>[3x]GAMGMNTPPELDTVLQAPYAYNWPTSKNVKIASRIGIPYSTFQTIQPVSDAPNNGIGQITFNQPLGNLTGGAPRLRVSFTAEIKNILADSSLKDQIGLKSFPVNRSIPVAVINMNGKTFTSYPAQLIKLHQYNADPLELALLSPCSDVDEYNKIKAVSMNNPYRQ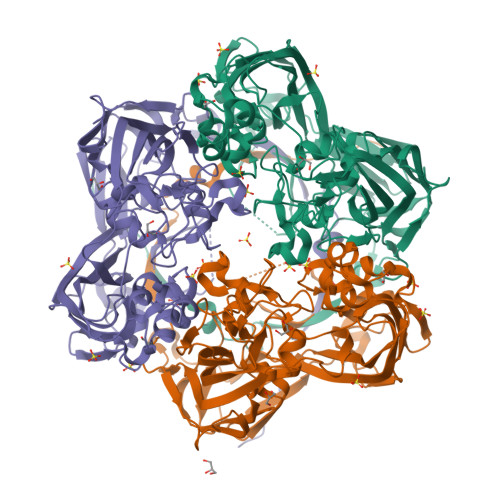GTESTDSRMSRGLGCNYAYYIHPRAAGSTSVKIDFVVDEALVANPTQYKNIKDPVPFRNLNTFKVILDGQFKPENMIGIADDVKLVAGKADFEVDITGFKINMLVQNWVAPLEIGDIPKTIIYNTPLISLEGNISSMCLNTKDPYGIPGERNKHILTTHSMAMNNVPSMFAVMVSQETPTKKFAPDQLAGIIGLEIKVDSDVGIFRELEQQQLYELSSSNGYNKRFSCFSGALANGLTVADPAVAAGNKFKEAIFGAGSVIFFRPSDLGLKDYNVMANANKSINMQVQATFVTPEAAGTGAHYKLEVFSIRDNLTYSFEDGTFMDDLTLYTPDQLLRSPLKLTDDNNKLMRVMGG>IVGGYTCQENSVPYQVSLNSGYHFCGGSLINDQWVVSAAHCYKSRIQVRLGEHNINVLEGNEQFVNAAKIIKHPNFDRKTLNNDIMLIKLSSPVKLNARVATVALPSSCAPAGTQCLISGWGNTLSSGVNEPDLLQCLDAP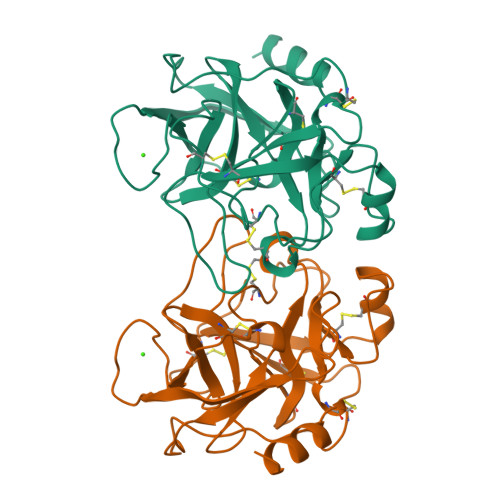LLPQADCEASYPGKITDNMVCVGFLEGGKSSCQGDSGGPVVCNGELQGIVSWGYGCALPDNPGVYTKVCNYVDWIQDTIAAN[2x]>MGSDKIHHHHHHMPKIWTERIFDDPEIYVLRIDDDRIRYFEAVWEIPEGISYNAYLVKLNGANVLIDGWKGNYAKEFIDA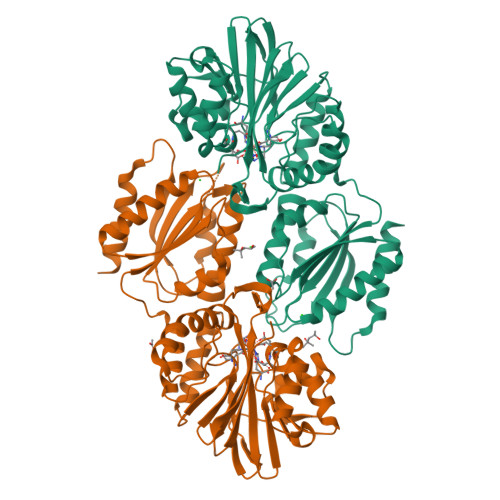LSKIVDPKEITHIIVNHTEPDDSGSLPATLKTIGHDVEIIASNFGKRLLEGFYGIKDVTVVKDGEEREIGGKKFKFVMTPWLHWPDTMVTYLDGILFSCDVGGGYLLPEILDDSNESVVERYLPHVTKYIVTVIGHYKNYILEGAEKLSSLKIKALLPGHGLIWKKDPQRLLNHYVSVAKGDPKKGKVTVIYDSMYGFVENVMKKAIDSLKEKGFTPVVYKFSDEERPAISEILKDIPDSEALIFGVSTYEAEIHPLMRFTLLEIIDKANYEKPVLVFGVHGWAPSAERTAGELLKETKFRILSFTEIKGSNMDERKIEEAISLLKKELE[2x]>[2x]MAGNECPELQPPVHGKIEPSQAKYFFKDQVLVSCDTGYKVLKDNVEMDTFQIECLKDGTWSNKIPTCKIVDCRAPGELEHGLITFSTRNNLTTYKSEIKYSCQEPYYKMLNNNTGIYTCSAQGVWMNKVLGRSLPTCLPECGQPSRSLPSLVQRIIGGRNAEPGLFPWQALIVVEDTSRVPNDKWFGSGALLSASWILTA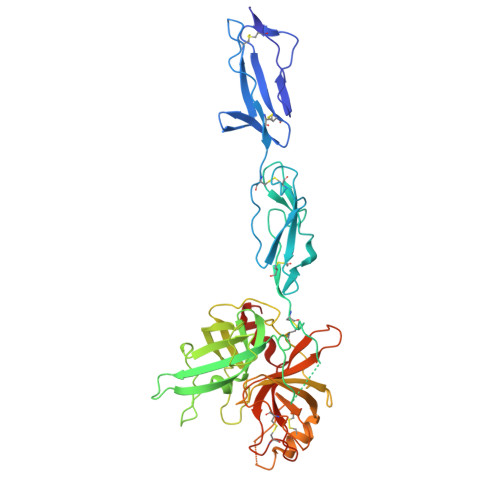AHVLRSQRRDTTVIPVSKEHVTVYLGLHDVRDKSGAVNSSAARVVLHPDFNIQNYNHDIALVQLQEPVPLGPHVMPVCLPRLEPEGPAPHMLGLVAGWGISNPNVTVDEIISSGTRTLSDVLQYVKLPVVPHAECKTSYESRSGNYSVTENMFCAGYYEGGKDTCLGDSGEAFVIFDDLSQRWVVQGLVSWGGPEECGSKQVYGVYTKVSNYVDWVWEQMGLPQSVVEPQVER> MSNLLTVHQNLPALPVDATSDEVRKNLMDMFRARQVFSEHTWKMLLSVCRSWAAWCKLNNRKWFPAEPEDVRDYLLYLQARGLAVKTIQQHLGQLNMLHRRSGLPRPSDSNAVSLVMRRIRKENVD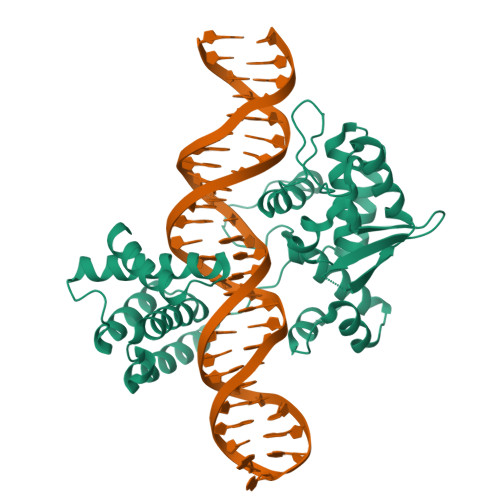AGERAKQALAFERTDFDQVRSLMENSDRCQDIRNLAFLGIAYNTLLRIAEIARIRVKDISRTDGGAMLIHIGRTKTLVSTAGVEKALSLGVTKLVERWISVSGVADDPNNYLFCRVRKNGVAAPSATSQLSTRALEGIFEATHRLIYGAKDDSGQRYLAWSGHSARVGAARDMARAGVSIPEIMQAGGWTNVNIVMNYIRNLDSETGAMVRLLEDGD>MATATEQWVLVEMVQALYEAPAYHLILEGILILWIIRLLFSKTYKLQERSDLTVKEKEELIEEWQPEPLVPPVPKDHPALNYNIVSGPPSHKTVVNGKECINFASFNFLGLLDNPRVKAAALASLKKYGVGTCGPRGFYGTFDVHLDLEDRLAKFMKTEEAIIYSYGFATIASAIPAYSKRGDIVFVDRAACFAIQKGLQASRSDIKLFKHNDMADLERLLKEQEIEDQKNPRKARVTRRFIVVEGLYMNTGTICPLPELVKLKYKYKARIFLEESLSFGVLGEHGRGVTEHYGINIDDIDLISANMENALASIGGFCCGRSFVIDHQRLSGQGYCFSASLPPLLAAAAIEALNIMEENPGIFAVLKEKCGQIHKALQGISGLKVVGESLSPAFHLQLEESTGSREQDVRLLQEIVDQCMNRSIALTQARYLEKEEKCLPPPSIRVVVTVEQTEEELERAASTIKEVAQAVLL[2x];>MRPEPGGCCCRRTVRANGCVANGEVRNGYVRSSAAAAAAAAAGQIHHVTQNGGLYKRPFNEAFEETPMLVAVLTYVGYGVLTLFGYLRDFLRYWRIEKCHHATEREEQKDFVSLYQDFENFYTRNLYMRIRDNWNRPICSVPGARVDIMERQSHDYNWSFKYTGNIIKGVINMGSYNYLGFARNTGSCQEAAAKVLEEYGAGVCSTRQEIGNLDKHEELEELVARFLGVEAAMAYGMGFATNSMNIPALVGKGCLILSDELNHASLVLGARLSGATIRIFKHNNMQSLEKLLKDAIVYGQPRTRRPWKKILILVEGIYSMEGSIVRLPEVIALKKKYKAYLYLDEAHSIGALGPTGRGVVEYFGLDPEDVDVMMGTFTKSFGASGGYIGGKKELIDYLRTHSHSAVYATSLSPPVVEQIITSMKCIMGQDGTSLGKECVQQLAENTRYFRRRLKEMGFIIYGNEDSPVVPLMLYMPAKIGAFGREMLKRNIGVVVVGFPATPIIESRARFCLSAAHTKEILDTALKEIDEVGDLLQLKYSRHRL[2x];>MAGMALARAW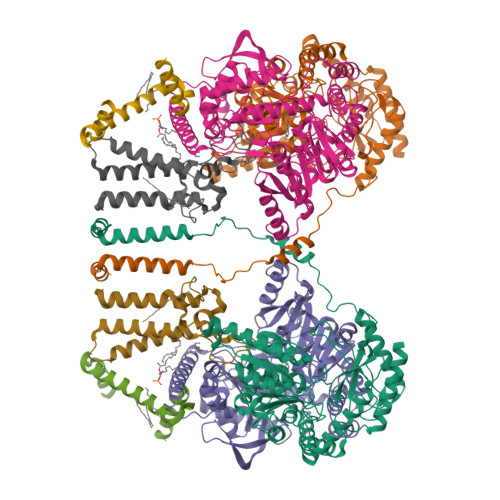KQMSWFYYQYLLVTALYMLEPWERTVFNSMLVSIVGMALYTGYVFMPQHIMAILHYFEIVQ[2x];>MNVGTAHSEVNPNTRVMNSRGIWLSYVLAIGLLHIVLLSIPFVSVPVVWTLTNLIHNMGMYIFLHTVKGTPFETPDQGKARLLTHWEQMDYGVQFTASRKFLTITPIVLYFLTSFYTKYDQIHFVLNTVSLMSVLIPKLPQLHGVRIFGINKY[2x]>[12x]MAQDALSDGFVRLCIDPSLNFFGEGCKILVEGQITDDATAAENVVTCVNSELDLVERFGQGSVLTESLRKVFCMCKSGVSVYALPRADAAAAVSAVYTLTVTGTALTDGRVQLYMGEAEYSLDIGVDEGDTPTQIAAKIVAAISPDFPYEATAAAGVITLTARNGGTIGNHLSVIYTNLGSCTSVTPEGVTVAFAQTTPGSVNPEPNDYASVVNECCFAVYVLSSDDTDWQENLRDWIRSAWDCSKPQCFGHGYVFNKGTLGQVLADGDNSAELSRLALPTTYPVLPYLTNAAYGALSACSTCENPELNVQGQTYGLLSCINMPESCTP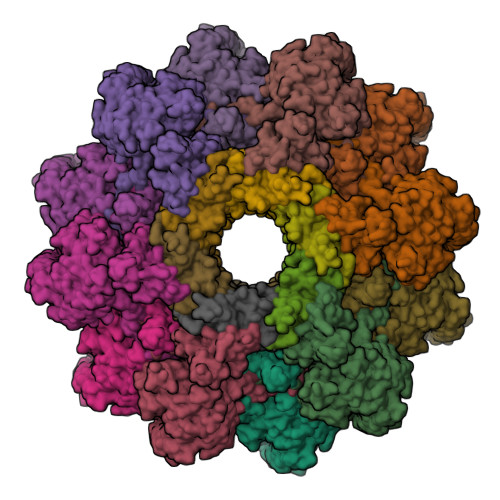GWEFTEVTQLQNNGFVVSGPATTSGQGNFTSPYIYNDVTNYLRDEKNRPNATFRDASSRRLAAATGVALATFLQQFNGLAVFTKNTNIKTGIIGTNLRLMLGKIRKWASDNVGVLFSEFDNINEDIQLVSDFDVQPKCVGQPGVFHLNMRYRPPVRGARINVNLVPALFDNCDR;>MACNKQNGVKNILITFTHCDTGEVIGPISHEQPDDTLPTYKTCAWTNTALTNGAVMRSASNATMTLPVVRDPRVPLAWYQGCAQIDAQVEKFDGTVMTLTEGAVTEPEESDGRAVTMTIIAAEIDELLPPGSLAAA[12x]> MSRIDDLQQDIESLLSEINSLEESREKLKAKIKDKRKNEESANPIVQEFEDLFDQFPQLNNFLFNEHPELEETDDKDISRAQADIPATPIPYEPKKRAKLENEEILPEQEWVLKTQPMVQHQMFDPGVADLLDTDILTSPSKRKRKLKIDDISTSDRSELEDYIVLENVYRMFGITFFPLVDPIDLKIKDASGEIFVDREMLGIRLEVFSERTSQFEKPHYVLLKKRIKSNSWFLFKHTIPSFIDVQGIFDDTNGGLVISHDDAYLFAKRVFLQLVEVQKRRQIFKDLEAKKIIHDLDLDLESSMVSFFVKDIKVELFVKQNEIVSCSILDDIHDFSQNNKSKWEIALLGSLDDLELKLNHSFATIFK;> MDFTSDTTNSHDTSNSHLSLEDAVGTHHAGEADVNIDGDEKQQLSLLDDDQVRALKLQEEKDALLTRRNTLLQEIQTYQNILMKENNSKTKNGDILQNDITQDFLNLISISSSNPNSAISDRKRVERINGLTNLQKELVTKYDTLPLLNMNLRLSYLRDHTYPHLQVSVQSRDRVHNDGIEVLVVNYKFCRNTMNPFEIQFKMFYKFEDSTLLKWEILRISTNVRLKAKQLLATRNFQKCLLSLYEFDKIKSKKTGIFQNLINLLKRKTRCYLMNNSDSLIVERVIREGRLTTIKLQINFIITMPGERGKPRNCFLPMSKISIALWKGGERFNQIDLDEICYGLIKEYGVKTGLKEICNVCLFPDMYAR;> MAADRDNFLQNIENDSINNGQAMDLSPNRSSSESDSSILMNVNDIKTLRLDVAPEAKSTQSKKSLFYENSDDAEEGEIEERTNKEEGQYHHKGSKQLRFEVGKESTGKLQSHLSDGSATSGEGNVRPWEFRKVIQAEYRERLPRNYELKHWKKPSKIMIGSILRLLETNTVSALDSVFEKYEKEMNQMTHGDNNEVKRIYSKKERLLEIILTKIKKKLRQAKFPSRISERDLDIEYIYSKRQFIQNRYSQELQNNERLEAILSREQNLLEETRKLCMNLKTNNKKRLTEKLIQKDLHPVLNKAMEYTYGLESTNGFMHPDGPVTFRNDSHELNLMLNDPIKSTADVRLDKEEVLSLLPSLKEYTKKSKELKETMGQMISDSHEEEIKEVFVPHHESHQDKTEEDIH;> MDRDTKLAFRLRGSHSRRTDDIDDDVIVFKTPNAVYREENSPIQSPVQPILSSPKLANSFEFPITTNNVNAQDRHEHGYQPLDAEDYPMIDSENKSLISESPQNVRNDEDLTTRYNFDDIPIRQLSSSITSVTTIDVLSSLFINLFENDLIPQALKDFNKSDDDQFRKLLYKLDLRLFQTISDQMTRDLKDILDINVSNNELCYQLKQVLARKEDLNQQIISVRNEIQELKAGKDWHDLQNEQAKLNDKVKLNKRLNDLTSTLLGKYEGDRKIMSQDSEDDSIRDDSNILDIAHFVDLMDPYNGLLKKINKINENLSNELQPSL;> MTDTYNSISNFIENELTALLSSDDYLMDDLAGELPNEVCRLLKAQVIEKRKDAMSRGKQDLLSKEIYDNESELRASQSQQIMELVGDIPKYSLGSELRNRVEGEPQSTSIERLIEDVLKLPQMEVADEEEVEVENDLKVLSEYSNLRKDLILKCQALQIGESKLS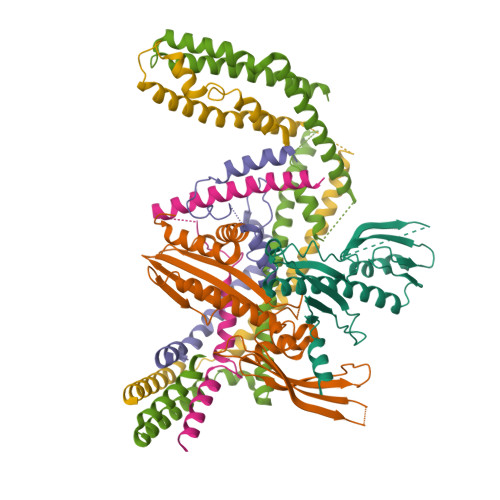DILSQTNSINSLTTSIKEASEDDDISEYFATYNGKLVVALEEMKLLLEEAVKTFGNSPEKREKIKKILSELKK;> MNSEQLLHNYVSDSLLTTLISFQEFKQQLQSYTSDEQQLQHWYELLQARDARVTSELEARIKQFFITLRSRLLRFLESEQLSHSLSLETLIDALYKINDLLQQRLQILDDAIQEKTSELAEFENMVRSPSAGDNAIPGLLQIIQSYINLLEEN>[2x]GSMKW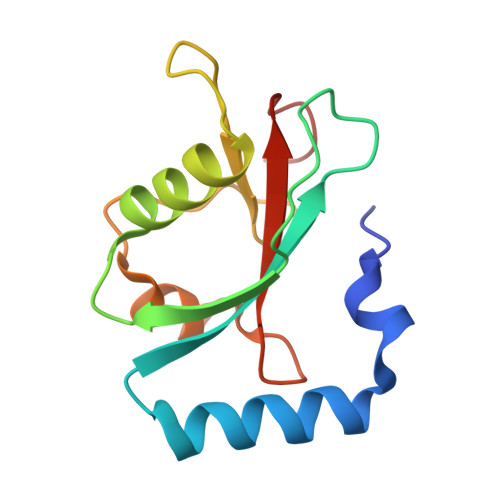MFKEDHSLEHRCVESAKIRAKYPDRVPVIVEKVSGSQIVDIDKRKYLVPSDITVAQFMWIIRKRIQLPSEKAIFLFVDKTVPQSSLTMGQLYEKEKDEDGFLYVAYSGENTFGF>MDNQKGRISIALLPFLAHGHISPFFELAKQLAKRNCNVFLCSTPINLSSIKDKDSSASIKLVELHLPSSPDLPPHYHTTNGLPSHLMLPLRNAFETAGPTFSEILKTLNPDLLIYDFNPSWAPEIASSHNIPAVYFLTTAAASSSIGLHAFKNPGEKYPFPDFYDNSNIIPEPPSADNMKLLHDFIACFERSCDIILIKSFRELEGKYIDLLSTLSDKTLVPVGPLVQDPMGHNEDPKTEQIINWLDKRAESTVVFVCFGSEYFLSNEELEEVAIGLEISTVNFIWAVRLIEGEKKGILPEGFVQRVGDRGLVVEGWAPQARILGHSSTGGFVSHCGWSSIAESMKFGVPVIAM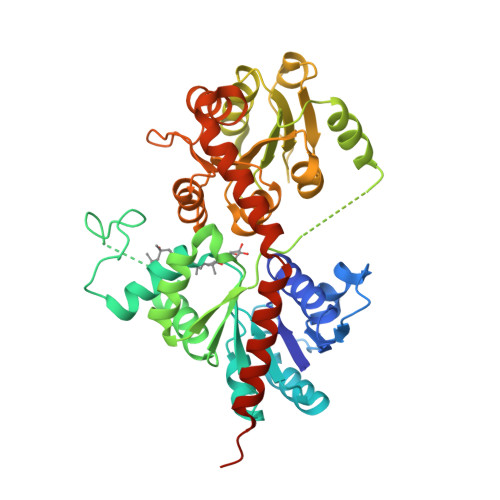ARHLDQPLNGKLAAEVGVGMEVVRDENGKYKREGIAEVIRKVVVEKSGEVIRRKARELSEKMKEKGEQEIDRAVEELVQICKKKKDEQENLYFQGHHHHHH[2x]>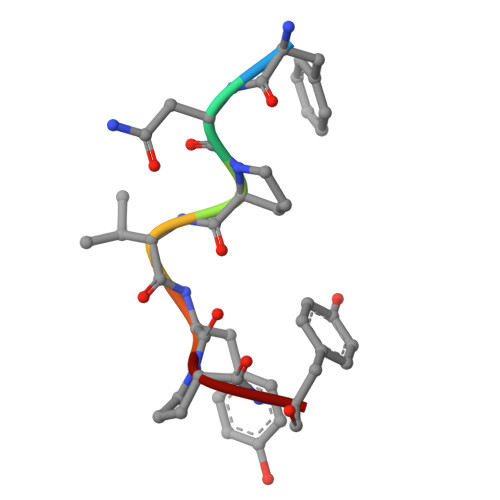 FNPVYPY> ARSTNTFNYATYHTLDEIYDFMDLLVAEHPQLVSKLQIGRSYEGRPIYVLKFSTGGSNRPAIWIDLGIHSREWITQATGVWFAKKFTEDYGQDPSFTAILDSMDIFLEIVTNPDGFAFTHSQNRLWRKTRSVTSSSLCVGVDANRNWDAGFGKAGASSSPCSETYHGKYANSEVEVKSIVDFVKDH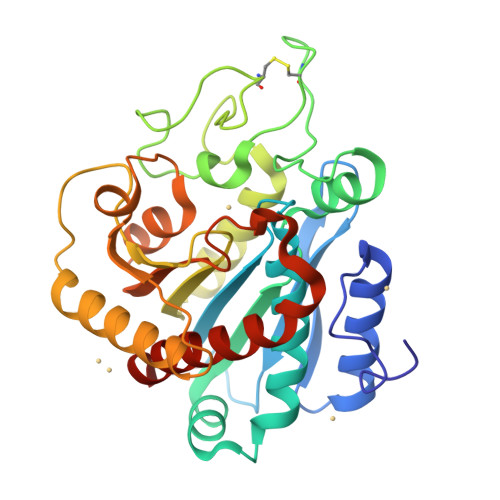GNFKAFLSIHSYSQLLLYPYGYTTQSIPDKTELNQVAKSAVAALKSLYGTSYKYGSIITTIYQASGGSIDWSYNQGIKYSFTFELRDTGRYGFLLPASQIIPTAQETWLGVLTIMEHTVNNLY>[2x]SHMFSDCRFGSVT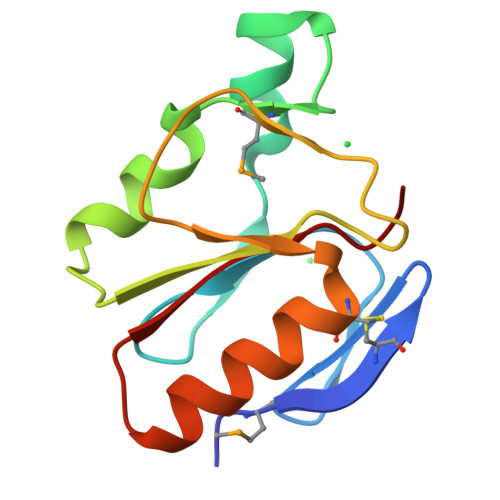YRGREYRSDIVVHVDGSVTPRRKEISRRKYGTSHVMAEEELEELLEEKPESIIIGSGVHGALETGFRSDATVLPTCEAIKRYNEERSAGRRVAAIIHVTC> EYIKLKVIGQDSSEIHFKVKMTTHLKKLKESYCQRQGVPMNSLRFLFEGQRIADNHTPKELGMEEEDV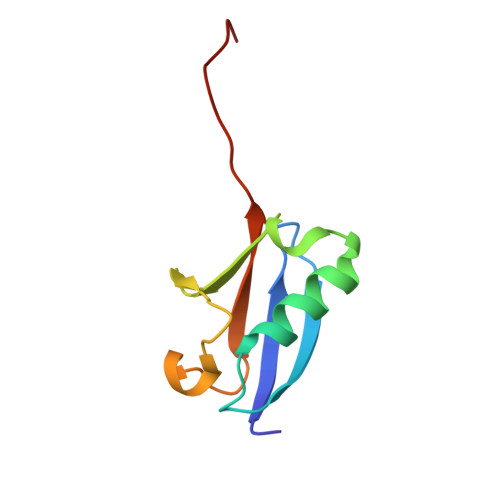IEVYQEQTGGHSTVC> MKEITFKINGQEMIVPEGTTILEAARMNNIDIPTLCYLKDINEIGACRMCLVEIAGARALQAACVYPVANGIEVLTNSPKVREARRVNLELIL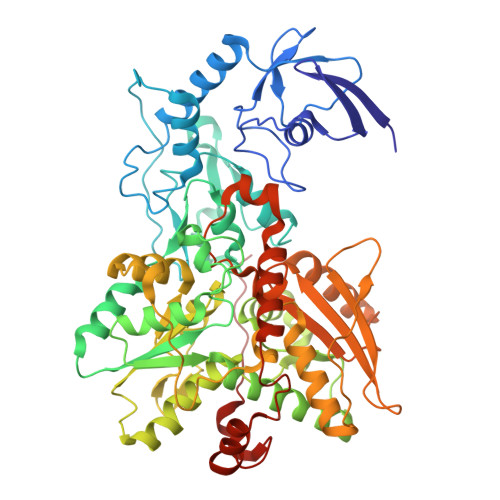SNHNRECTTCIRSENCELQTLATDLGVSDIPFEGEKSGKLIDDLSTSVVRDESKCILCKRCVSVCRDVQSVAVLGTVGRGFTSQVQPVFNKSLADVGCINCGQCIINCPVGALKEKSDIQRVWDAIADPSKTVIVQTAPAVRAALGEEFGYPMGTSVTGKMAAALRRLGFDKVFDTDFGADVCIMEEGTELIGRVTNGGVLPMITSCSPGWIKFIETYYPEAIPHLSSCKSPQNITGALLKNHYAQTNNIDPKDMVVVSIMPCTAKKYEVQREELCTDGNADVDISITTRELARMIKEARILFNKLPDEDFDDYYGESTGAAVIFGATGGVMEAAVRTVADVLNKKDIQEIDYQIVRGVDGIKKASVEVTPDLTVNLVVAHGGANIREVMEQLKAGELADTHFIELMACPGGCVNGGGQPIVSAKDKMDIDIRTERAKALYDEDANVLTYRKSHQNPSVIRLYEEYLEEPNSPKAHHILHTKYSAKPKLV>[2x]MAFPKRLEYGGHALVWSGDWSAAGARKAIAGAARAGYDYIEIALLDPWQIDVALTKDLLQEYNLRAHASLGLSAATDVTSTDPAIVAKGDELLRKATDVLYALGGSELCGVIYCALGKYPGPASRENRANSVAAMQRLADYAADKGINIDLEVVNRYETNIMNTGLEGLAFLDEVNRPNAFLHLDT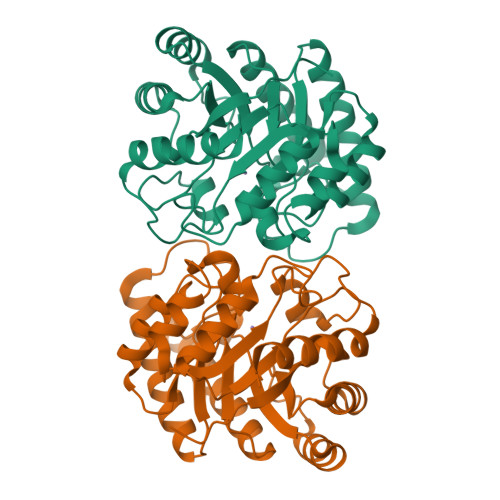YHMNIEENGMAKSVLAAGDRLGYVHIGESHRGYLGTGNVDFASFFAALKQIDYRGPITFESFSSEIVDPKLSNTLCVWRNLWHDSDDLAGKALEFIKQRYGSHHHHHH ACETIC ACID SALICYLOYL-AMINO-ESTER | C9 H9 N O4 | 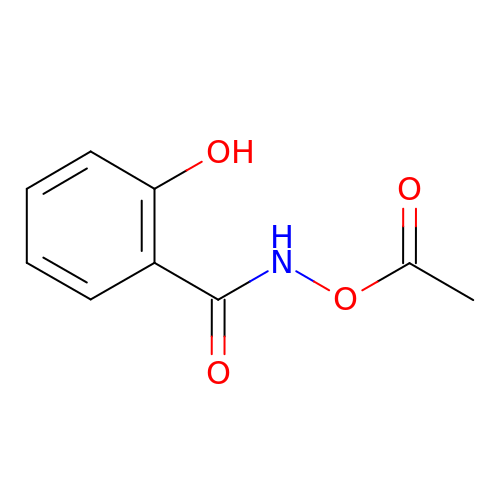PCFWLDHLJWUGSU-UHFFFAOYSA-N> MG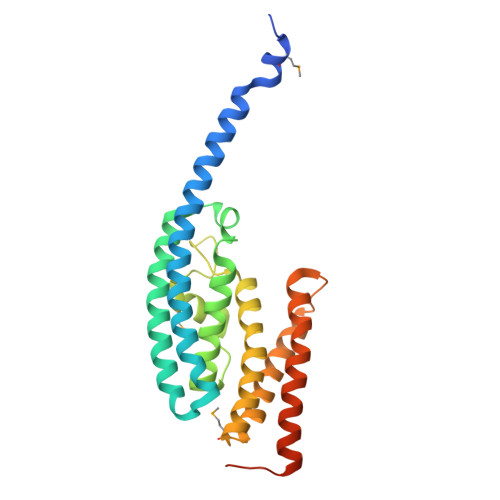SSHHHHHHSQDPMSNFVNLDIFSNYQKYIDNEQEVRENIRIVVREIEHLSKEAQIKLQIIHSDLSQISAACGLARKQVELCAQKYQKLAELVPAGQYYRYSDHWTFITQRLIFIIALVIYLEAGFLVTRETVAEMLGLKISQSEGFHLDVEDYLLGILQLASELSRFATNSVTMGDYERPLNISHFIGDLNTGFRLLNLKNDGLRKRFDALKYDVKKIEEVVYDVSIRGLSSKEKDQQEEPAVPATE> HLVCPMSKSPYVDPHKSGHEIWEEFSMSFTPAVKEVVEFAKRI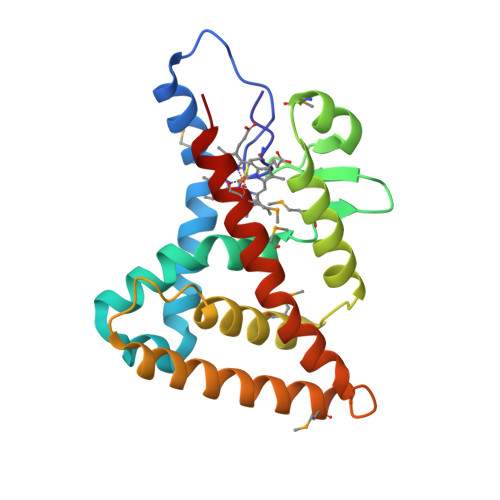PGFRDLSQHDQVNLLKAGTFEVLMVRFASLFDAKERTVTFLSGKKYSVDDLHSMGAGDLLNSMFEFSEKLNALQLSDEEMSLFTAVVLVSADRSGIENVNSVEALQETLIRALRTLIMKNHPNEASIFTKLLLKLPDLRSLNNMHSEELLAFKVHP>[5x]GQDMVSPPPPIADEPLTVNTGIYLIECYSLDDKAETFKVNAFLSLSWKDRRLAFDPVRSGVRVKTYEPEAIWIPEIRFVNVENARDADVVDISVSPDGTVQYLERFSARVLSPLDFRRYPFDSQTLHIYLIVRSVDTRN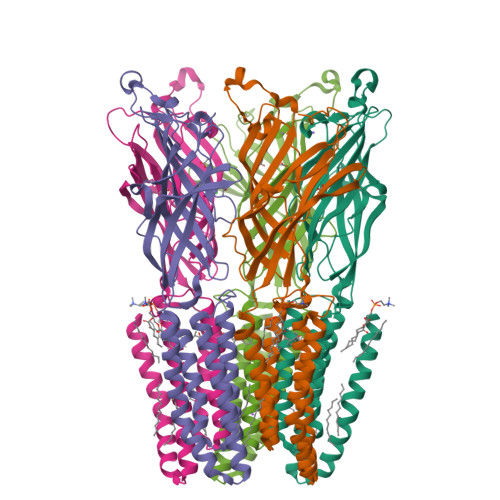IVLAVDLEKVGKNDDVFLTGWDIESFTAVVKPANFALEDRLESKLDYQLRISRQYFSYIPNIILPMLFILFISWTAFWSTSYEANVTLVVSTLIAHIAAAILVETNLPKTPYMTYTGAIIFMIYLFYFVAVIEVTVQHYLKVESQPARAASITRASRIAFPVVFLLANIILAFLFFGF GRKs chiefly function to initiate the deactivation of agonist occupied GPCRs primarily through phosphorylation of their cytoplasmic C-terminal tails, which leads to the recruitment of arrestins and ultimately clathrin-mediated endocytosis. Individual GRKs are validated targets for the treatment of human conditions ranging from heart failure to diabetes. Although GRK2 has thus far been the primary focus of drug discovery efforts, GRK5 has been increasingly targeted as a potential treatment for cardiac hypertrophy. The development of inhibitors selective for GRK5 over GRK2 has been challenging due to high sequence identity in their active sites.

GRK1 was used as a surrogate for GRK5 because the structure of GRK5 has not yet been reported, GRK1 is known to readily crystallize in various ligand states, and GRK1 is a relatively close homolog of GRK5 with 47% sequence identity. The GRK1·amlexanox crystal structure was solved to 2.8 Å spacings and has four similar but non-identical complexes in the asymmetric unit. The largest conformational variation observed among them occurs in the active site tether (AST) loop that passes over the active site, which is disordered in one chain. Amlexanox exhibits strong omit map density in the active site of each monomer where its 2-aminopyridine group forms hydrogen bonds to backbone atoms of hinge residues Thr265, and Met267 in a manner similar to that observed in other reported GRK·inhibitor and adenine nucleotide complexes. Its tricyclic ring system sandwiched between the side chains of Leu193, Val201, and Ala214 in the small lobe and the carbonyl of Met267 and the side chain of Leu321 in the large lobe. However, unlike previously reported GRK inhibitors, amlexanox does not form extensive interactions with the P-loop. Instead, the long axis of the drug extends out to form hydrophobic interactions with the AST loop in 3 of the 4 chains with its isopropyl group. This binding mode is similar to that of GSK2163632A in complex with GRK1, wherein a large aromatic system of the compound packs primarily along the hinge and forms extensive interactions with the AST. The GRK1 amlexanox crystal structure demonstrates that the drug binds directly in the active site of the kinase in a manner that mimics the adenine ring of ATP. Although a larger panel of kinases would have to be evaluated in order to know how promiscuous amlexanox is, its ability to inhibit diverse kinases likely reflects its structural similarity to adenine, in that in only forms hydrogen bonds to backbone atoms and that it occupies the same flat, aromatic binding pocket in the active site.

>[4x]MDFGSLETVVANSAFIAARGSFDASSGPASRDRKYLARLKLPPLSKCEALRESLDLGFEGMCLEQPIGKRLFQQFLRTHEQHGPALQLWKDIEDYDTADDALRPQKAQALRAAYLEPQAQLFCSFLDAETVARARAGAGDGLFQPLLRAVLAHLGQAPFQEFLDSLYFLRFLQWKWLEAQPMGEDWFLDFRVLGRGGFGEVFACQMKATGKLYACKKLNKKRLKKRKGYQGAMVEKKILAKVHSRFIVSLAYAFETKTDLCLVMTIMNGGDIRYHIYNVDEDNPGFQEPRAIFYTAQIVSGLEHLHQRNIIYRDLKPENVLLDDDGNVRISDLGLAVELKAGQTKTKGYAGTPGFMAPELLLGEEYDFSVDYFALGVTLYEMIAARGPFRARGEKVENKELKQRVLEQAVTYPDKFSPASKDFCEALLQKDPEKRLGFRDGSCDGLRTHPLFRDISWRQLEAGMLTPPFVPDSRTVYAKNIQDVGAFSTVKGVAFEKADTEFFQEFASGTCPIPWQEEMIETGVFGDLNVWRPDGHHHHHH>MDNYQELAIQFAAQAVDRNEIEQWVREFAYQGFDARRVIELLKQYGGADWEKDAKKMIVLALTRGNKPRRMMMKMSKEGKATVEALINKYKLKEGNPSRDELTLSRVAAALAGRTCQALVVLSEWLPVTGTTMDGLSPAYPRHMMHPSFAGMVDPSLPGDYLRAILDAHSLYLLQFSRVINP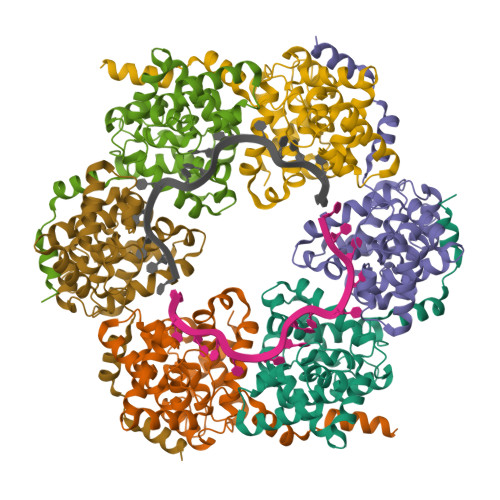NLRGRTKEEVAATFTQPMNAAVNSNFISHEKRREFLKAFGLVDSNGKPSAAVMAAAQAYKTAA[3x]> MAATAAEAVASGSGEPREEAGALGPAWDESQLRSYSFPTRPIPRLSQSDPRAEELIENEEPVVLTDTNLVYPALKWDLEYLQENIGNGDFSVYSASTHKFLYYDEKKMANFQNFKPRSNREEMKFHEFVEKLQDIQQRGGEERLYLQQTLNDTVGRKIVMDFLGFNWNWINKQQGKRGWGQLTSNLLLIGMEGNVTPAHYDEQQNFFAQIKGYKRCILFPPDQFE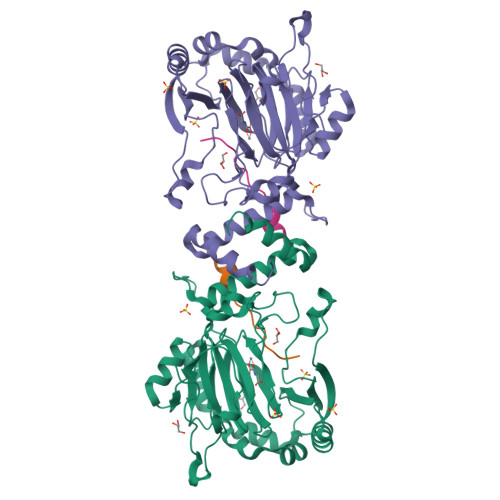CLYPYPVHHPCDRQSQVDFDNPDYERFPNFQNVVGYETVVGPGDVLYIPMYWWHHIESLLNGGITITVNFWYKGAPTPKRIEYPLKAHQKVAIMRNIEKMLGEALGNPQEVGPLLNTMIKGRYN;> NIAIERRQGDIAALLIAAGADVNAHAK(2R)-2-{4-[3-(4-{[(2R)-2-hydroxy-3,3-dimethylbutyl]oxy}-3-methylphenyl)pentan-3-yl]-2-methylphenoxy}butane-1,4-diol | C29 H44 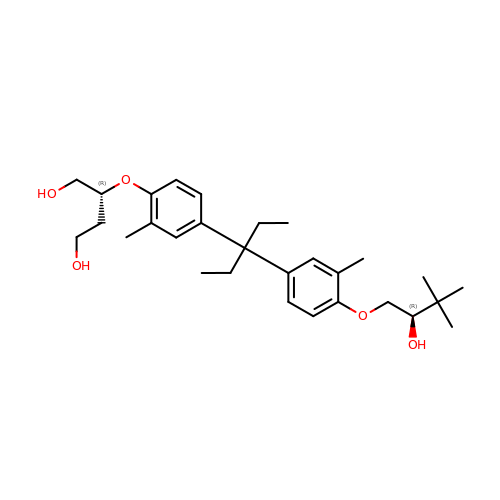O5 | DKNLNQKPISQAEP-SQHAQQRYSA-N> MVPISPIETVPVKLKPGMDGPKVKQWPLTEEKIKALVEICTELEKEGKISKIGPENPYNTPVFAIKKKNSTRWRKLVDFRELNKRTQDFWEVQLGIPHPAGLKKKKSVTVLDVGDAYFSVPLDEDFRKYTAFTIPSINNETPGIRYQYNVLPQGWKGSPAIFQSSMTKILEPFKKQNPDIVIYQYMDDLYVGSDLEIGQHRTKIEELRQHLLRWGLYTPDQKHQKEPPFLWMGYELHPDKWTVQPIVLPEKDSWTVNDICKLVGKLNWASQIYPGIKVRQLSKLLRGTKALTEVIPLTEEAELELAENREILKEPVHGVYYDPSKDLIAEIQKQGQGQWTYQIYQEPFKNLKTGKYARMRGAHTNDVKQLTEAVQKITTESIVIWGKTPKFKLPIQKETWETWWTEYWQATWIPEWEFVNTPPLVKLWYQLEKEPIVGAETFYVDGAANRETKLGKAGYVTNKGRQKVVPLTNTTNQKTELQAIYLALQDSGLEVNIVTDSQYALGIIQAQPDKSESELVNQIIEQLIKKEKVYLAWVPAHKGIGGNEQVDKLVSAGIRKVL;> PISPIETV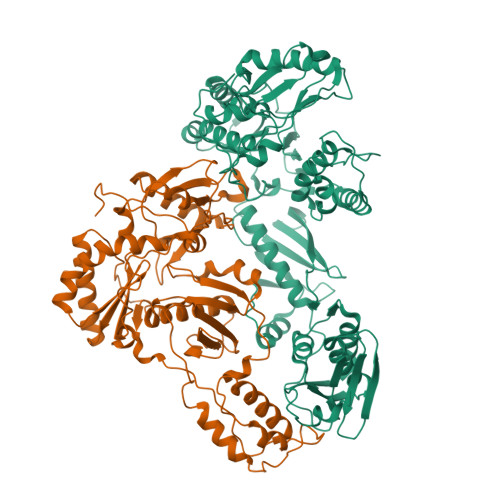PVKLKPGMDGPKVKQWPLTEEKIKALVEICTEMEKEGKISKIGPENPYNTPVFAIKKKDSTKWRKLVDFRELNKRTQDFWEVQLGIPHPAGLKKKKSVTVLDVGDAYFSVPLDEDFRKYTAFTIPSINNETPGIRYQYNVLPQGWKGSPAIFQSSMTKILEPFKKQNPDIVIYQYMDDLYVGSDLEIGQHRTKIEELRQHLLRWGLTTPDKKHQKEPPFLWMGYELHPDKWTVQPIVLPEKDSWTVNDIQKLVGKLNWASQIYPGIKVRQLSKLLRGTKALTEVIPLTEEAELELAENREILKEPVHGVYYDPSKDLIAEIQKQGQGQWTYQIYQEPFKNLKTGKYARMRGAHTNDVKQLTEAVQKITTESIVIWGKTPKFKLPIQKETWETWWTEYWQATWIPEWEFVNTPPLVKLWYQGGHHHHHHH>MQEKSITIATEGGYAPWNFSGPGGKLDGFEIDLANALCEKMKAKCQIVAQNWDGIMPSLTGKKYDAIMAAMSVTPKRQEVIGFSIPYAAGINGFAVMGDSKLAEMPGLGETYSLDSQADAAKKAIADISSFLNGTTVGVQGSTTASTFLDKYFKGSVDIKEYKSVEEHNLDLTSGRLDAVLANATVLAAAIEKPEMKGAKLVGPLFSGGEFGVVAVGLRKEDTALKADFDAAIKAASEDGTIKTLSLKWFKVDVTPQHHHHHH[2x]

Two Agrobacterium ABC-transporters and their cognate periplasmic binding proteins (PBPs) OccJ and NocT import octopine and nopaline/octopine, respectively. Recognition and import of opines are conferred by periplasmic binding proteins (PBPs) and their associated ATP-binding cassette (ABC) transporters. The PBP OccJ is associated with the octopine transporter of octopine-type A. tumefaciens while NocT is associated with nopaline uptake in the nopaline-type A. tumefaciens. OccJ shares 47% sequence identity with NocT and belongs to cluster F within the PBP structural classification.

The X-ray structures of the unliganded and liganded OccJ with octopine were solved at 2.35 and 2 Å resolution respectively. The liganded crystal contained two very similar molecules in the asymmetric unit as indicated by the overall root mean square deviations (RMSD) for all Cα atoms of 0.28 Å. The liganded form adopts a closed conformation whereas the unliganded form adopts an open conformation. The octopine bound between the two closed lobes of OccJ is very well defined in the electron density maps, and is surrounded by 18 residues defining the ligand binding site of OccJ. In OccJ, the pyruvate moiety interacts with four non-conserved side chains: Ser91, Asn111, Thr163 and Asn202, which correspond to Gly97, Met117, Ser169 and Ser207 in NocT. Ser91 in OccJ once again appears as a major difference in the binding site of the pyruvate moiety of octopine in OccJ compared with NocT, making this residue potentially critical for octopine binding. Indeed, Ser91 in OccJ plays a remarkable role in holding octopine in three parts of the molecule, including both carboxyl groups. OccJ displays a high selectivity and nanomolar range affinity for octopine. Here, we established a structural basis for the high octopine specificity of the PBP OccJ and defined the high affinity octopine binding signature in which five residues form the binding signature of the octopine ketoacid: Ser91-Asn111-Thr163-Ala164-Asn202.> GSHMKPHPWFFGKIPR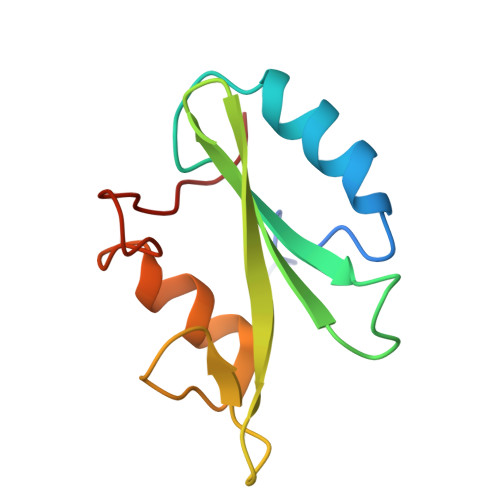AKAEEMLSKQRHDGAFLIRESESAPGDFSLSVKFGNDVQHFKVLRDGAGKYFLWVVKFNSLNELVDYHRSTSVSRNQQIFLRDIE(2S)-3-{4-[2-(4-{[(2R)-2-hydroxy-3,3-dimethylbutyl]oxy}-3-methylphenyl)propan-2-yl]-2-methylphenoxy}propane-1,2-diol 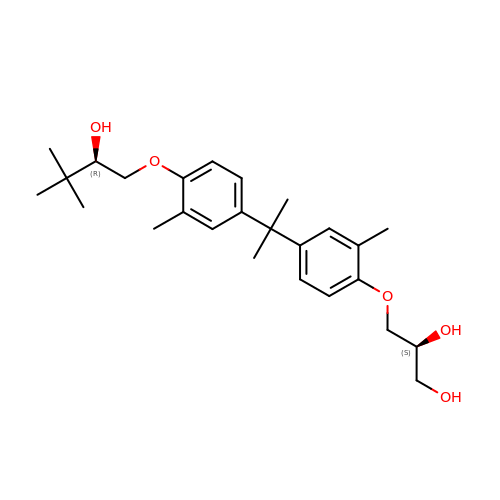| C26 H38 O5 | QOQDEYISGNGHKZ-URXFXBBRSA-N>[4x]MDPEQIKTALGSGLLSFPVTHFDAEGRFAADSYREHVEWLAGYKAPVLFAAGGTGEFFSLKPDEIPTIVAAAKEVAGETAIVSGCGYGTEIAVDIARSVEKVGADGILLLPHYLIDAPQEGLYAHIKKVCQSVGIGVMVYNRDNSVLQADTLARLCDECPNLVGFKDGTGDIGLVR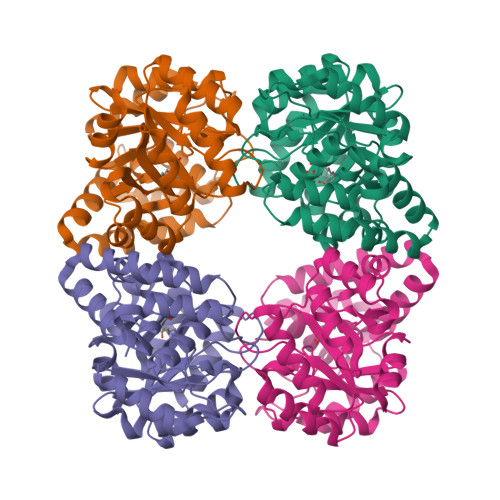QITAKMGDRLMYLGGMPTAELFAEAYLGAGFTTYSSAVFNFVPGLANEFYAALRAGERATCERILVDFFYPFMAIRNRAKGYAVSAVKAGVRLQGFNAGPVRAPLKDLTNEEIGMLEALIGTHKRKAWSHPQFEK> MIDEALFDAEEKMEKAVAVARDDLSTIRTGRANPGMFSRITIDYYGAATPITQLASINVPEARLVVIKPYEA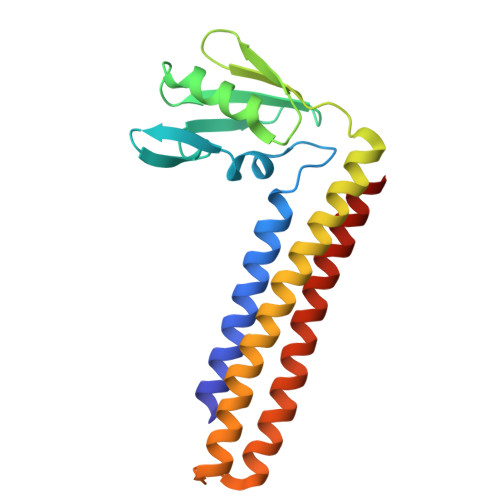NQLRAIETAIRNSDLGVNPTNDGALIRVAVPQLTEERRRELVKQAKHKGEEAKVSVRNIRRKAMEELHRIRKEGEAGEDEVGRAEKDLDKTTHQYVTQIDELVKHKEGELLEV> MNINQLILRNLKKNLRNYYLYVFALIFSVALYFAFVTLQYDPAINEVKASIKGAAAIKTASILLVAVVAIFILYANTIFIKRRSKEIGLFQLIGMTKHKIFRILSAENVMLYFGSLAIGVAAGFSISKLVLMILFKIVDVKADAKLHFSEQALVQTVIVFCGIYLLIMIMNYTFIKKQSILSLFKVTSSTEDKVKKISFFQMLIGALGIVLILTGYYVSSELFGGKFKTINELFVAMSFILGSVIIGTFLFYKGSVTFISNIIRKSKGGYLNISEVLSLSSIMFRMKSNALLLTIITTVSALAIGLLSLAYISYYSSEKTAEQNVAADFSFMNEKDAKLFENKLRESNISFVKKATPVLQANVDIANIMDGTPKEMQGDPGNMQLAVVSDKDVKGVDVAAGEAVFSGYTDLLQKIMVFKDSGVIKVKSKHETQPLKYKGLREEFLVSYTFTSGGMPAVIVDDSLFKQLDKDKDPRIQLAQSTFIGVNVKHDDQMEKANELFQQVNKKNEHLSRLDTSAAQKSLFGMVMFIVGFLGLTFLITSGCILYFKQMGESEDEKPSYTILRKLGFTQGDLIKGIRIKQMYNFGIPLVVGLFHSYFAVQSGWFLFGSEVWAPMIMVMVLYTALYSIFGFLSVLYYKKVIKSSL;>MSGHHHHHHVILEANKIRKSYGNKLNKQEVLKGIDIHIEKGEFVSIMGASGSGKTTLLNVLSSIDQVSHGTIHINGNDMTAMKEKQLAEFRKQHLGFIFQDYNLLDTLTVKENILLPLSITKLSKKEANRKFEEVAKELGIYELRDKYPNEISGGQKQRTSAGRAFIHDPSIIFADEPTGALDSKSASDLLNKLSQLNQKRNATIIMVTHDPVAASYCGRVIFIKDGQMYTQLNKGGQDRQTFFQDIMKTQGVLGGVQHEH[2x];>MIKAFLIERRSWIAAFLFQQALMLFIAFVDPSISFGNVLYMVYLCILFFIIFLWFRYRKETAFYKSLKTWENNLDVTAINEPETPFEAMVERSIAGQTEHLKQTAARHRLALENEKDELMAWIHEVKTPLTAMHLIIDRMEEKALKSQLSYEWLRIHLLLDQQLHQKRISFIENDLSVEFIQLQPLIFKEIKDLQSWCIQKGIGFDIQLEAKEVLSDAKWLAFIIRQLLTNAVKYSEASEIEIKSFQKGEQTQLQVKDCGRGIDPKDVPRIFDKGFTSTTDHHDQASTGMGLYLAKKAAAPLLIHIDVESEFGAGTVFTLTFPIRNQFEHVISV[2x]

One such mechanism widely found across Firmicute bacteria involves antimicrobial peptide sensing and resistance membrane protein complexes collectively known as Bce modules. These modules are composed minimally of an ATP-binding cassette (ABC) transporter which defends against antimicrobial peptides without transport across the membrane, and an interacting two-component system containing a sensor histidine kinase and response regulator. In this module bceA encodes the ATPase domains, bceB encodes the membrane-spanning permease domain of the ABC transporter BceAB, and bceS encodes the histidine kinase that phosphorylates the response regulator encoded by bceR. Previous studies have established that BceAB mediates resistance against bacitracin, likely by freeing bacitracin from the lipid target undecaprenyl-pyrophosphate (UPP). To understand this critical membrane protein interaction and the molecular details underpinning the Bce module flux-sensing mechanism, we have determined the cryo-EM structure of the complete BceAB-S complex from B. subtilis in nucleotide-free and ATPγS-bound states.

To understand how BceS interacts with BceB in the transmembrane region, we combined all particles that displayed clear secondary structure for TM helices in 3D classification and refined these particles into a single volume. Residual signal subtraction focused on the TM region was followed with a round of 3D classification without alignment, generating two distinct classes of particles with high-resolution features in the TM region. Refinement of these two classes independently produced separate 3D volumes each at ~3.4 Å overall resolution. We refer to these two reconstructions as TM-state-1 and TM-state-2. The overall structure of the BceAB-S complex in TM-state-1 and TM-state-2 is nearly identical (overall RMSD ~ 0.6 Å), with very minor shifts in the position of TM helices. Within the detergent belt 14 total TM helices were clearly identified, with 10 belonging to BceB and another 4 belonging to the BceS dimer. Although the buried protein surface area between BceB and BceS is relatively small, we identified several lipid-like densities between BceB and BceS TM helices within the bilayer plane. Nevertheless, our cryo-EM structures clearly demonstrate that most of the interaction between BceB and BceS is mediated through protein-lipid interactions rather than direct protein–protein interaction.N-({5-[4-(2-amino-4-oxo-4,7-dihydro-1H-pyrrolo[2,3-d]pyrimidin-6-yl)butyl]thiophen-2-yl}carbonyl)-L-glutamic acid | C20 H23 N5 O6 S | 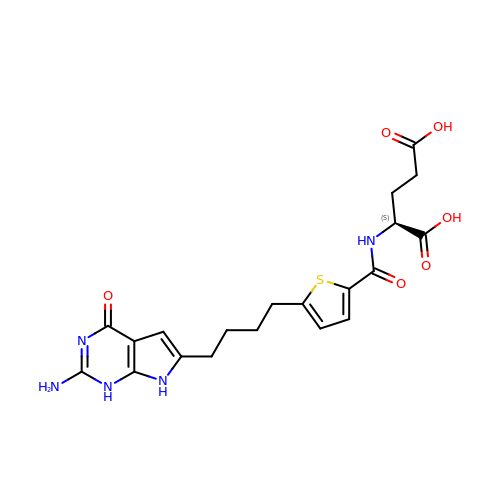ADFLVKAWSSGDBU-ZDUSSCGKSA-N>[2x]GSHMYKSVNITFELDERIDKVLNEKCSAYTVELGTEVNEFACVVADA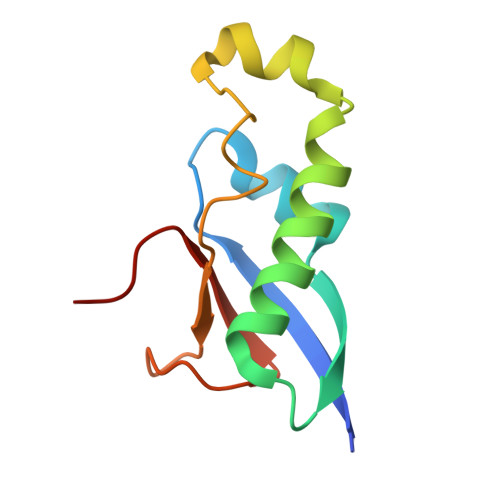VIKTLQPVSELLTPLGIDLDEWSMATYYLFDESGEFKLASHMYCSFYPPDE Receptor tyrosine kinases exhibit a variety of activation mechanisms despite highly homologous catalytic domains. Here, we show that the juxtamembrane (JM) segment enhances RET catalytic domain activity through Y687. Structure-function analyses identified interactions between the JM hinge, αC helix, and an unconventional activation-loop serine phosphorylation site that engages the HRD motif and promotes phospho-tyrosine conformational accessibility and regulatory spine assembly. We demonstrate that this phospho-S909 arises from an intrinsic RET dual-specificity kinase activity and show that an equivalent serine is required for RET signaling in Drosophila.

We have determined two similar crystal structures of a construct containing the RET JM region and KD (amino acids 659–1013) at 3.3 and 2.95 Å, respectively. Both crystal structures contained the PP1 tyrosine kinase inhibitor in the nucleotide-binding pocket, had an ordered proximal portion of the RET JM segment, and had a hyper-phosphorylated status with four sites phosphorylated (Y809, Y905, S909, and Y928). The structures differ slightly in resolution and in the occupancy of the phospho-S909 site. In the crystal structures presented in this study, phospho-S909 displaces phospho-Y905 and adopts an approximate equivalent position by engaging activation segment residues R897 and R912, as well as R873 from the HRD motif instead. In this situation, Y905 does not engage the side chain of the αC helix R770; as a consequence, phospho-Y905 projects away from the body of the RET kinase to mimic a fully solvent-accessible conformer. The second unexpected phosphorylation site at Y928 is positioned beneath the tethered phospho-S909 and is likely to further disrupt interactions of phospho-Y905 with the activation loop. Phospho-Y928 forms hydrogen bonds with side chains of R873 (HRD motif) and activation loop R897 at the top and with H926 from beneath. The JM-KD structure revealed contacts from a short segment of the proximal JM region (residues D707 to W717) with a hydrophobic patch composed of residues from different structural elements including β4 (L790), β5 (L800, L801, L802), and αC helix (L769, L772, L773, F776, L779). Examination of the crystal structure revealed that in RET the R-spine is composed of four hydrophobic residues originating from the αF helix connecting N- and C-lobes; these residues include H872 (from the catalytic HRD motif), F893 (from the DFG motif), L779 (αC helix), and L790 (β-4 strand). W717 caps from the top the R-spine in a linear tetrad compatible with an active DFG in conformation of the kinase.

> CYHKFAHKPPISSAEMTFRRPAQAFPVSYSSSGARRPSLDSMENQVSVDAFKILEDPKWEFPRKNLVLGKTLGEGEFGKVVKATAFHLKGRAGYTTVAVKMLKENASPSELRDLLSEFNVLKQVNHPHVIKLYGACSQDGPLLLIVEYAKYGSLRGFLRESRKVGPGYLGSGGSRNSSSLDHPDERALTMGDLISFAWQISQGMQYLAEMKLVHRDLAARNILVAEGRKMKISDFGLSRDVYEEDSYVKRSQGRIPVKWMAIESLFDHIYTTQSDVWSFGVLLWEIVTLGGNPYPGIPPERLFNLLKTGHRMERPDNCSEEMYRLMLQCWKQEPDKRPVFADISKDLEKMMVKRR> MDEIVKNIREGTHVLLPFYETLPELNLSLGKSPLPSLEYGANYFLQISRVNDLNRMPTDMLKLFTHDIMLPESDLDKVYEILKI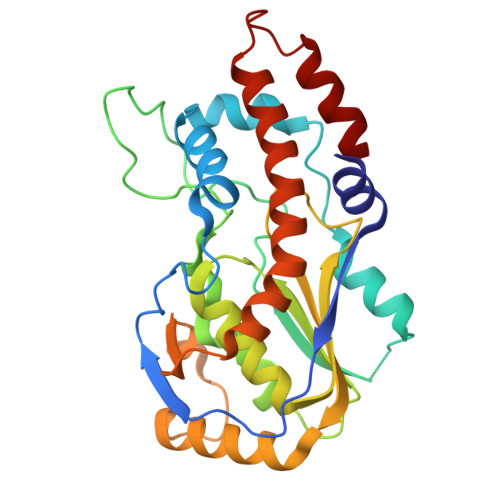NSVKYYGRSTRADAVVADLSARNKLFKRERDAIKSNNHLTENNLYISDYKMLTFDVFRPLFDFVNEKYCIIKLPTLFGRGVIDTMRIYCSLFKNVRLLKCVSDSWLKDSAIMVASDVYKKNLDLFMSHVKSVTKSSSWKDVNTVQFSILNDPVDTEFINKFLEFSNRVYEALYYVHSLLYSSMTSDSKSIENKHQRRLVKLLL>MSFTVVIPARYQSTRLPGKPLADIGGKPMIQWVYEQAMQAGADRVIIATDDERVEQAVQAFGGVVCMTSPNHQSGTERLAEVVAKMAIPADHIVVNVQGDEPLIPPAIIRQVADNLAACSAPMATLAVEIEDEAEVFNPNAVKVITDKSGYALYFSRATIPWDRDNFAKADKAIVQPLLRHIGIYAYRAGFINTYLDWQPSQLEKIECLEQLRVLWHGEKIHVAVALEAPPAGVD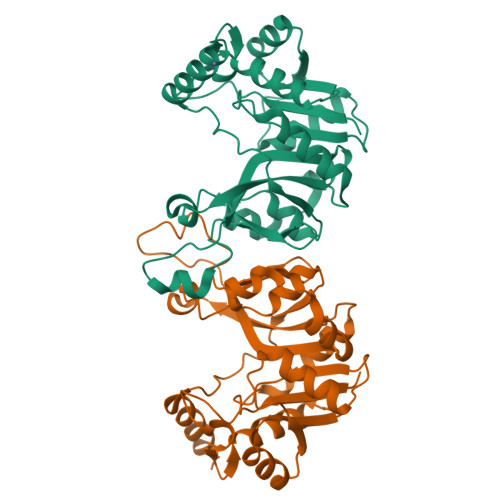TPEDLEVVRRIVAERAQ[4x]>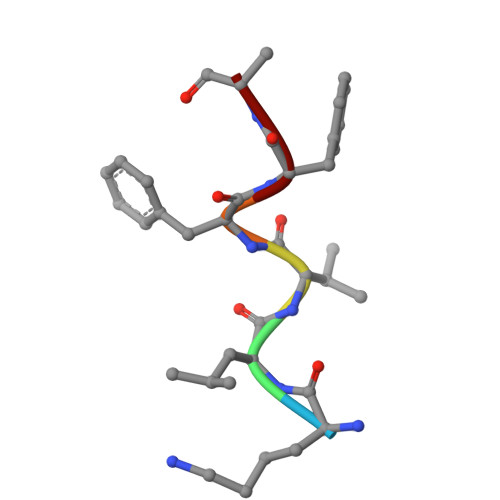 KLVFFA2-(1-PIPERIDINYL)-1,3-THIAZOL-4-AMINE | C8 H13 N3 S | 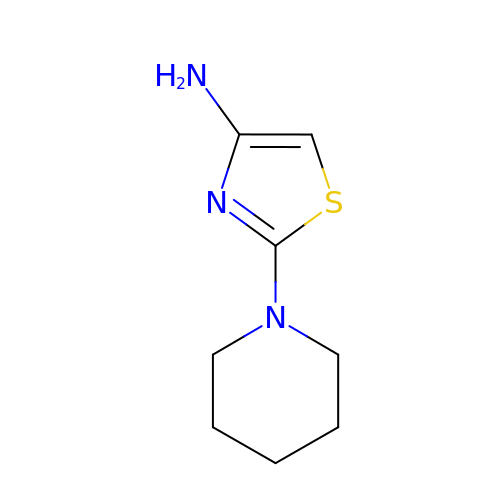UXCNXLNTJSYWJW-UHFFFAOYSA-N> GAMEPLTASMLASAPPQEQKQMLGERLFPLIQAMHPTLAGKITGMLLEIDNSELLHML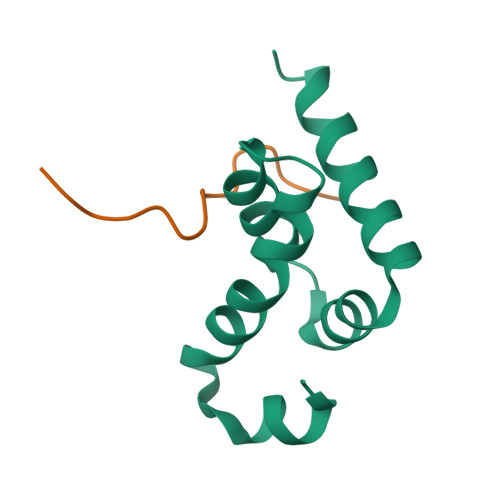ESPESLRSKVDEAVAVLQAHQAKE;> ELNPNAEVWGAPVLH>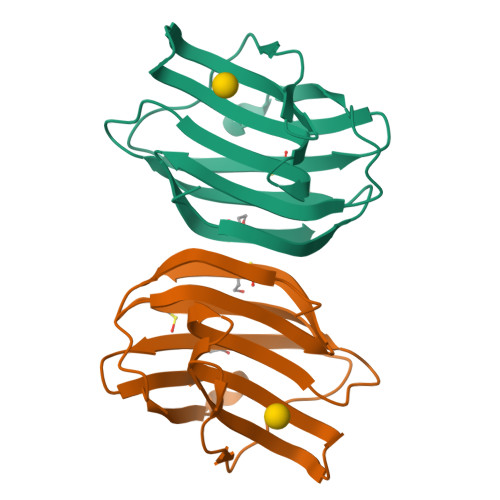ACGLVASNLNLKPGECLRVRGEVAPDAKSFVLNLGKDSNNLCLHFNPRFNAHGDANTIVCNSKDGGAWGTEQREAVFPFQPGSVAEVCITFDQANLTVKLPDGYEFKFPNRLNLEAINYMAADGDFKIKCVAFD[2x]>[2x]GGMGNNSRASNPVPLEDQIGALLGEHPRQIVPLHAGRRAQVLRCHFQDGHSVIVKSFTEVAETTRGEWDALRFLAAHVPAIAPRPLARSKDRRLVAMEDLRGETLARLLERESEAGARRP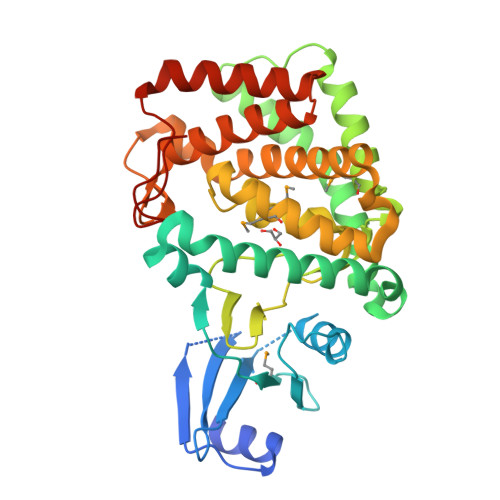LVRIADALGHLHGAQAPRVDGLPRALRDEYRKQADECVALRGKVRALLGRAGVEPTPGFDGAWLELVERMGSPGPFLTFTHGDLAPSNVLLTDDGPRLLDFEYTGARSALYDVMFWEAVVPFPRSLARPMTQAYRRALASHLPAARDDARFRRELLTLKTHRFFWWLTFRLDEALAGGDAHWVPGWRLRPAYLFYLQNYVSTARRLGARGPLLKTAQALSSRLRRGWKERAGYPDHFLGKLKPPGP> GGAGUAGAAGCGUUCAGCGGCCGAAAGGCCGCCCGGAAAUUGCU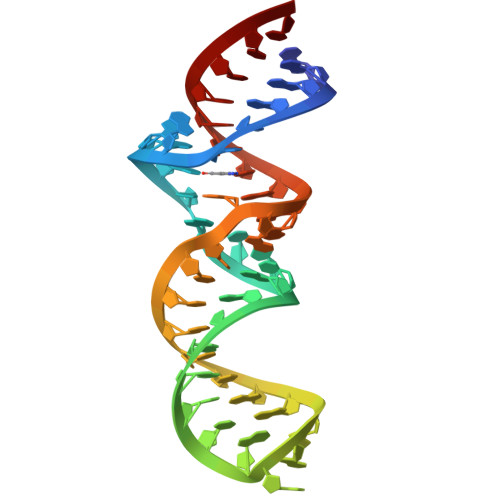CC>[4x]MGRLDGKVIILTAAAQGIGQAAALAFAREGAKVIATDINESKLQELEKYPGIQTRVLDVTKKKQIDQFANEVERLDVLFNVAGFVHHGTVLDCEEKDWDF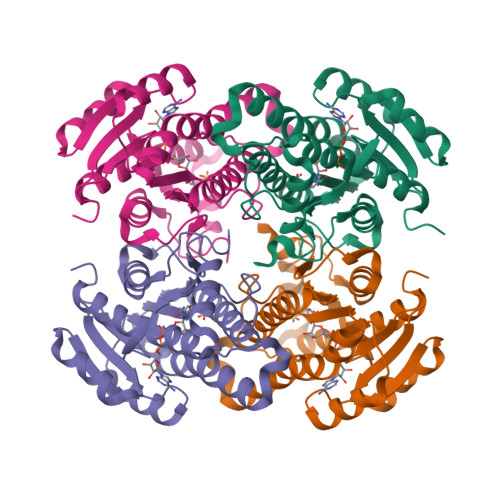SMNLNVRSMYLMIKAFLPKMLAQKSGNIINMSSVASSVKGVVNRCVYSTTKAAVIGLTKSVAADFIQQGIRCNCVCPGTVDTPSLQERIQARGNPEEARNDFLKRQKTGRFATAEEIAMLCVYLASDESAYVTGNPVIIDGGWSLG> QSEEYCASAWVGIDGDTCETAILQTGVDFCYEDGQTSYDAWYEWYPDYAYDFSDITISEGDSIKVTVEATSKSSGSATVENLTTGQSVTHTFSGNVEGDLCETNAEWIVEDFESGDSLVA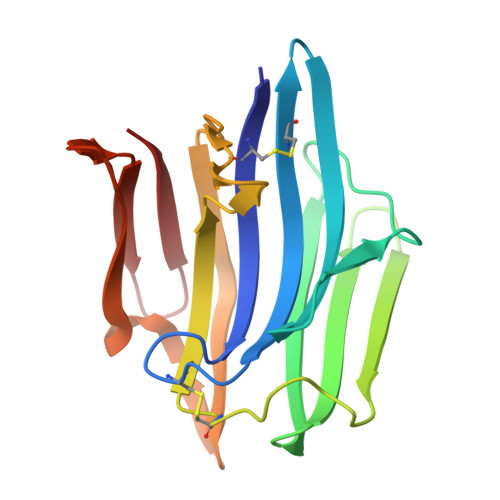FADFGSVTFTNAEATSGGSTVGPSDATVMDIEQDGSVLTETSVSGDSVTVTYV>[2x]MKHHHHHHPMTTKQWGITPPISTAPATEQENALNTALINELKNQNLFESPAESEKRVKVLDELQQITTEFVKKVSLAKHMNEKMANEAGGKIFTYGSYRLGVYGPGSDIDTLVVVPKHVSRDNFFQDLEPMLREREEVTDLAAVPDAYVPIIKFKFLGISIDLIFARLSVPRVPRDLELSDNNLLKGVEERCVLSLNGTRVTDQILQLVPNRAVFKHALRAIKFWAQRRAIYANVVGFPGGVAWAMMVARICQLYPNAVSSVIVAKFFRILHQWNWPQPILLKPIEDGPLQVRIWNPKLYPSDKAHRMPIITPAYPSMCATHNITLSTQTIILREMVRAGEIADQIMVKALPWSALFQKHDFFHRYKHYLTITAAAKTAEAQLKWAGLVESKLRHLVTRLELVDAIALAHPFNKGFDKVYNCSSEEEAQQVASGV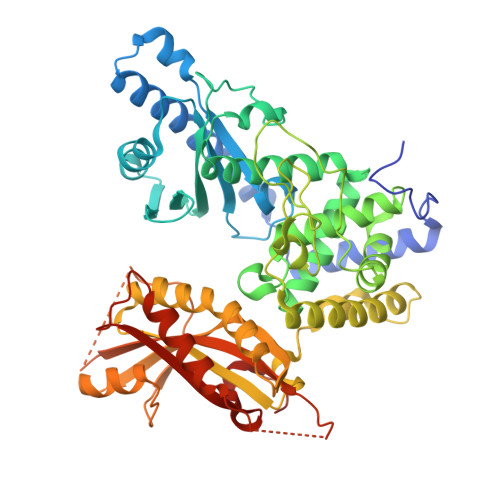TLEVAYESTDHEKLANDTVNEEKADNTESKADGSENGEKQIFPVYTTTCYIGLELEKKKGHPIKRLDISWPTQEFYELCKKWDKYDDTLMNVFIKNTKNTALPDEVFEPGEERPKA> KQYDR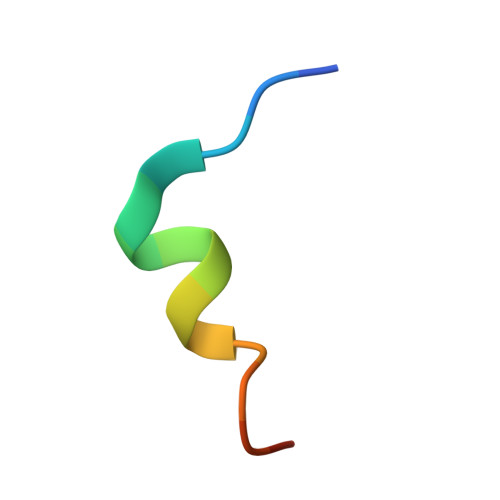EFLLDFQFMPA> RKVESSKVSKKR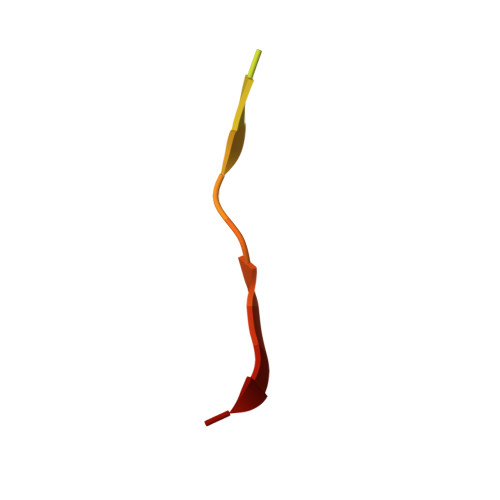IAPTPVYP> APLVHHHHHHALDENLYFQGALATTLDEADEAGKRIFGPRVGNELCEVKHVLDLCRIRESVSEELLQLEAKRQELNSEIAKLNLKIEACKKSIENAKQDLLQLKNVISQTEHSYKELMAQNQPKLSLPIRLLPEKDDAGLPPPKATRGCRLHNCFDYSRCPLTSGFPVYVYDSDQFVFGSYLDPLVKQAFQATARANVYVTENADIACLYVILVGEMQEPVVLRPAELEKQLYSLPHWRTDGHNHVIINLSRKSDTQNLLYNVSTGRAMVAQSTFYTVQYRPGFDLVVSPLVHAMSEPNFMEIPPQVPVKRKYLFTFQGEKIESLRSSLQEARSFEEEMEGDPPADYDDRIIATLKAVQDSKLDQVLVEFTCKNQPKPSLPTEWALCGEREDRLELLKLSTFALIITPGDPRLVISSGCATRLFEALEVGAVPVVLGEQVQLPYQDMLQWNEAALVVPKPRVTEVHFLLRSLSDSDLLAMRRQGRFLWETYFSTADSIFNTVLAMIRTRIQIPAAPIREEAAAEIPHRSGKAAGTDPNMADNGDLDLGPVETEPPYASPRYLRNFTLTVTDFYRSWNCAPGPFHLFPHTPFDPVLPSEAKFLGSGTGFRPIGGGAGGSGKEFQAALGGNVPREQFTVVMLTYEREEVLMNSLERLNGLPYLNKVVVVWNSPKLPSEDLLWPDIGVPIMVVRTEKNSLNNRFLPWNEIETEAILSIDDDAHLRHDEIMFGFRVWREARDRIVGFPGRYHAWDIPHQSWLYNSNYSCELSMVLTGAAFFHKYYAYLYSYVMPQAIRDMVDEYINCEDIAMNFLVSHITRKPPIKVTSRWTFRCPGCPQALSHDDSHFHERHKCINFFVKVYGYMPLLYTQFRVDSVLFKTRLPHDKTKCFKFI

The completed linker tetrasaccharide represents the point of bifurcation in GAG biosynthesis: either EXTL3 adds an α-linked GlcNAc and initiates HS polymerisation or one of two closely related CSGALNACTs adds a β-linked GalNAc and initiates CS polymerisation. We show that selection of the GAG chain type occurs at the priming step: CSGALNACTs are capable of initiating CS synthesis on all GAG attachment sites, whereas EXTL3 requires specific features in the core protein to initiate HS synthesis. Structure-function analysis reveals that acidic residues in the glycopeptide substrate and a basic exosite in EXTL3 are critical for specifying HS biosynthesis. Our results demonstrate that modification with CS occurs by default and must be overridden by EXTL3 to produce HS.

In order to explain these data mechanistically, we determined crystal structures of an EXTL3 dimer lacking the coiled-coil (residues 154–919) in the apo form (1.58 Å resolution) and with UDP and Mn2+ bound (2.10 Å resolution). The large dimer interface features an intermolecular disulfide bond (Cys793–Cys915) that staples the C-terminal tail of one subunit to the body of the other subunit. To determine whether basic residues are important for the selective modification of acidic acceptor glycopeptides, we mutated two pairs (K905A/R907A and K914A/K917A) and all five basic residues in the C-terminal tail of EXTL3 (5× mutant). All mutants assembled into disulfide-bonded dimers, suggesting that their folding was unaffected. The activity of these EXTL3 mutants was assessed with Tetra-BETA and TetraP-BETA as acceptor substrates. Mutation of Arg905 and Arg907 reduced conversion of TetraP-BETA to product by ≈60%, and mutation of all five basic residues resulted in an almost complete loss of activity. These effects were even more pronounced with Tetra-BETA as substrate, indicating that both the phosphate and the acidic residues in TetraP-BETA contribute to EXTL3 binding. We found that EXTL3 specificity is determined by a basic exosite >20 Å from the GlcNAc transferase site.Here, we report a general and rapid method for discovering α-helically constrained (Helicon) polypeptides that cooperatively induce the interaction between two target proteins without relying on previously known binders or an intrinsic affinity between the proteins. We show that Helicons are capable of binding every major class of E3 ubiquitin ligases, which are of great biological and therapeutic interest but remain largely intractable to targeting by small molecules. In addition to possessing increased stability and membrane permeability, Helicons are capable of binding large, flat protein surfaces that are inaccessible to targeting by small molecules, and Helicons have been developed to target a range of PPI targets in cells and in vivo. Characterizing Helicon-E3 co-structures and mechanisms of action, we identified new binding sites for α-helices on the E3 surfaces, as well as potential probes of the disease-linked E3, WWP123,24, highlighting the generality of our approach against this therapeutically important target class.

First, we focused on the NEDD4-like E3 ligases, which make up approximately a third of the HECT family. These include WWP1 and WWP2, which each consist of four tandem WW domains and a catalytic HECT domain at the C-terminus that transfers ubiquitin from a bound E2 first to itself and subsequently to the target substrate. We began by designing three HECT-containing protein constructs: a construct that stabilizes the autoinhibited, inactive state of WWP1 (WWP1WW-HECT), and WWP1/2 constructs that are able to adopt both the active and inactive conformations (WWP1HECT and WWP2HECT). The first profile (Group 1) represents Helicons such as those in cluster C71 (C71) that are pan-WWP-binders – binding indiscriminately to inactive and active forms of both HECT domains, which share ~70% sequence identity. We next solved the crystal structures of five Helicons, four in complex with WWP2HECT representing all three groups of HECT-binding clusters, and one from Group 1 with WWP1HECT. In all of the structures, we found that the HECT domains adopted similarly closed (inhibited) conformations. Group 1 Helicons H302 (WWP1HECT-binding) and H301 (WWP2HECT-binding) showed similar binding modes as each other, making contact only with the N-lobe of WWP1HECT or WWP2HECT, respectively.

> GSHMGFRWKLAHFRYLCQSNALPSHVKINVSRQTLFEDSFQQIMALKPYDLRRRLYVIFRGEEGLDYGGLAREWFFLLSHEVLNPMYCLFEYAGKNNYCLQINPASTINPDHLSYFCFIGRFIAMALFHGKFIDTGFSLPFYKRMLSKKLTIKDLESIDTEFYNSLIWIRDNNIEECGLEMYFSVDMEILGKVTSHDLKLGGSNILVTEENKDEYIGLMTEWRFSRGVQEQTKAFLDGFNEVVPLQWLQYFDEKELEVMLCGMQEVDLADWQRNTVYRHYTRNSKQIIWFWQFVKETDNEVRMRLLQFVTGTCRLPLGGFAELMGSNGPQKFCIEKVGKDTWLPRSHTCFNRLDLPPYKSYEQLKEKLLFAIEETE;> XDPASMRCHRAAHICSVLX> MEELTYRLFMVATVGMLAGTVFLLASSREVKPEHRRGVYISALVCGIAWYHYQKMGASWESGSYDTGLRYVDWVLTVPLMFVEVLAVTRKGAAYNEAVRNWGIAATVMIGAGYYGETSAAGSNEYWTGFVIAMATYVWLMRNLQAEGEGLKGDQAVAFENIKNLILVGWIIYPLGYIAPVVGDFDAIREVLYTIADIINKVGLGVLVLQMARVQSGEKVS

Here, we have functionally and structurally characterized a representative of the PR family found in a widely distributed clade of marine actinobacteria, Candidatus Actinomarina minuta, named MAR [marine actinobacterial rhodopsin or MacR (16)]. In summary, the sequence alignment and the photocycle measurements confirm that MAR is a member of the PR family, which functions as an outward proton pump at neutral and high pH. Overall, MAR consists of seven transmembrane helices, A to G, connected through short intracellular and extracellular loops. A retinal chromophore is covalently bound to Lys200 of helix G. The fold of the MAR is similar to that of other PRs.

Using the rose-form crystals, we obtained two different structures of the O state: under the proton-pumping (pH 8.4) and pumping-inhibited (pH 4.6) conditions at the 1.4- and 1.09-Å resolutions, respectively. We will refer to these structures as the O* and O states for clarity. At the same time, the extracellular part of MAR turns into an almost fully dehydrated region because of the FG-loop closure (a key role in this process is the formation of a hinge in helix F). It can be concluded that the structural and spectroscopic data of the rose form of MAR allow assigning this state to the late O intermediate. Apparently, the O state is trapped by the crystallization conditions in the rose-colored crystals. Fortunately, the O intermediate state of PRs harbors a retinylidene Schiff base with an all-trans retinal, allowing it to be trapped in the dark under certain crystallization conditions. Compared to the structures of the ground, M-like, and N states, in the O state structure, an additional water molecule w6 is incorporated in the HBC between Glu83 and the carbonyl group of Lys200. Glu83 and w6 acquire two conformations. In the first conformation, Glu83 makes an H-bond with Ser41 and w6. w6 is stabilized by Ser41 and w5. In the second conformation, both Glu83 and w6 break their bonds with Ser41. Unexpectedly, the His-Asp pair remains protonated in both O* and O state structures, as indicated by the H-bond (2.7 and 2.6 Å, respectively) between the residues.>[2x]MGEFEKRAKELIERAKKLNTPAAKVIEEALKLF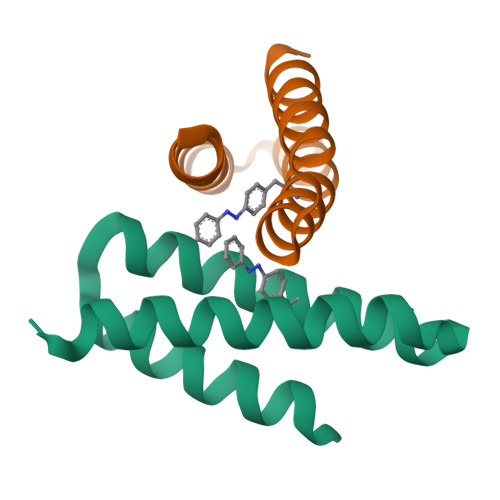IEAYKEAKKKGDALQQALLEESLAQAEEMLRRLEHHHHHH> MTRTTGTRTTGILADGAIRALFAGDKL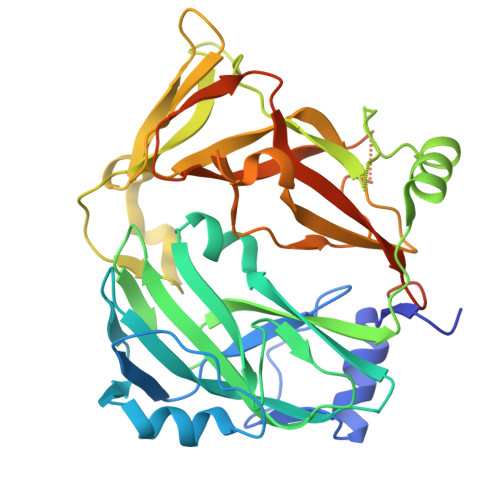KSEADLDVDQVQPASLDLRLGSKAYRVRASFMPGPGTRVIDKLNRFSLHEVDLSQGAVLETGCVYIVPLMESLALPADMSASANPKSSTGRLDIFTRVMTDNAQEFDKIPAGYTGPLYLEISPRTFPIVVRRGSRLSQIRFRIGHALLNESEVLKLHETETLVASENPNVTGGGIALSIDLKGFGENGLIGYRGKHHTAVVDVDKKAQHDVLDFWEPLFARGRAELILDPDEFYILVSREAVHVPPLYAAEMTPFDPLVGEFRVHYAGFFDPGFGHAQAGGTGSRAVLEVRSHEVPFILEHGQIVGRLVYEHMLEKPEGLYGTGLGSNYQAQGLKLSKHFRAE>[2x]GPGS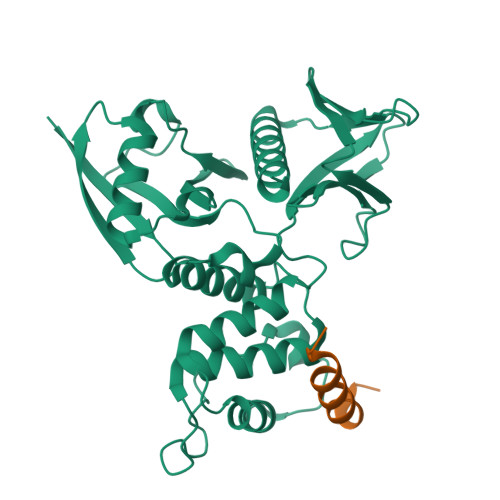MAGAIASRMSFSSLKRKQPKTFTVRIVTMDAEMEFNCEMKWKGKDLFDLVCRTLGLRETWFFGLQYTIKDTVAWLKMDKKVLDHDVSKEEPVTFHFLAKFYPENAEEELVQEITQHLFFLQVKKQILDEKIYCPPEASVLLASYAVQAKYGDYDPSVHKRGFLAQEELLPKRVINLYQMTPEMWEERITAWYAEHRGRARDEAEMEYLKIAQDLEMYGVNYFAIRNKKGTELLLGVDALGLHIYDPENRLTPKISFPWNEIRNISYSDKEFTIKPLDKKIDVFKFNSSKLRVNKLILQLCIGNHDLFMRRRKADSLEVQQ;>[2x]PKFGPYQKALREIRYSLLPFANESGTSAAAEV> TPEGLSSEQQRAFLAVTQTPHPAHLITGPAGTGKTTLLYALQEFYKGRAVTLAPTGTAALQARGQTVHSFFRFPA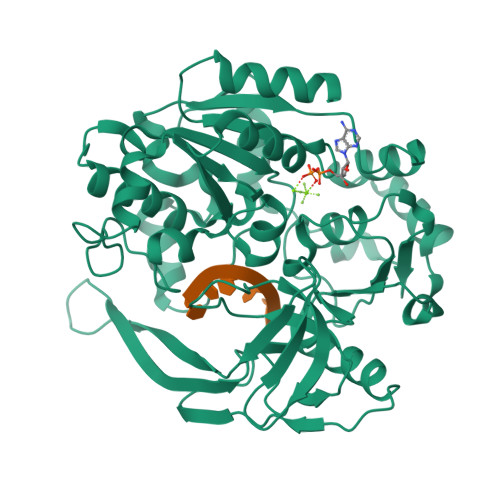RLLRYRHPEDIRPPGPHSPLRKAIEQMEVLILDEVGMVRVDLLEAMDWALRKTRKRLEEPFGGVKVLLLGDTRQLEPVVPGGEEALYIARTWGGPFFFQAHVWEEVALRVHRLWESQRQREDPLFAELLKRLRQGDPQALETLNRAAVRPDGGEEPGTLILTPRRKEADALNLKRLEALPGKPLEYQAQVKGEFAETDFPTEAALTLKKGAQVILLRNDPLGEYFNGDLGWVEDLEAEALAVRLKRNGRRVVIRPFVWEKIVYTYDSEREEIKPQVVGTFRQVPVRLAWALTVHKAQGLTLDKVHLELGRGLFAHGQLYVALTRVRRLQDLSLSRPIAPTELLWRPEVEVFETRIQEGIWQKSHGWPSL Cyclic nucleotide binding domains (CNB) confer allosteric regulation by cAMP or cGMP to many signaling proteins, including PKA and PKG. PKA of phylogenetically distant Trypanosoma is the first exception as it is cyclic nucleotide-independent and responsive to nucleoside analogues. Here, we show that natural nucleosides inosine, guanosine and adenosine are nanomolar affinity CNB ligands and activators of PKA orthologs of the important tropical pathogens Trypanosoma brucei, Trypanosoma cruzi, and Leishmania. Substitution of two to three amino acids in the binding sites is sufficient for conversion of CNB domains from nucleoside to cyclic nucleotide specificity.

To evaluate the binding mode, we solved the crystal structures of T. cruzi PKAR(200-503) and T. brucei PKAR(199-499) bound to inosine at 1.4 Å and 2.1 Å resolution, respectively. The structures of TbPKAR and TcPKAR show high overall similarity. Calculated RMSD of Cα alignment was 0.796 Å for the entire proteins and 0.281/0.342 Å for CNB-A and CNB-B, respectively. Residues that contribute to high affinity binding by interacting with the ribose moiety of inosine are identical in both structures and reside in a segment that we denoted ribose binding cassette (RBC), in analogy to the phosphate binding cassette (PBC) nomenclature for mammalian PKA. Likewise, the ‘capping’ by π-stacking with the purine ring in both sites (Y371/483TcPKAR, Y370/482TbPKAR) and the interacting residues in the lid-like αD helix are conserved. Residues G309; E310; E312 and A321 belong to Ribose Binding Cassette A (RBC-A), while G433; E434 and E436 are part of Ribose Binding Cassette B (RBC-B). Capping residues (Y371 and Y483) taking part in a π-stacking interaction with the hypoxanthine ring of inosine are marked with an asterisk. In the ligand-bound structures of TbPKAR and TcPKAR, this helix docks to theβ-barrel of the B-site, covers the binding pocket and shields the ligand from solvent. The high-resolution crystal structures of T. brucei PKAR and T. cruzi PKAR thus provides a molecular rationale for absence of binding and activation by cAMP.

> GRNRRRTVRSEGIDPEKAKLYQAPYFEKSEDEMNLITKLLTHNVLFSFLNTKDIKVVAGAMQRATFKHDDCIMEAGQTTCNKLYIIQSGHADIIKEGQKVYLKTEGTAVGELELMYDTPVVATVKVCTDELIAWVLDRDTYRNLVMGTAIRRRETYIQFLANVPFLGGLDSYEKLQLADALSSEEFSPGEYIIHYGEEGEWLYIIMEGTVEVIGRDADGEPTKVCEFTQGDHIGELEFLNNHRTVADVVATTHVITAKLNRRHFEMCLGPVIDVLKRCADDPKYEYYQNVLKTGAAQPSYVDDV> MIVSSSIVFDIFNYIGIVAFA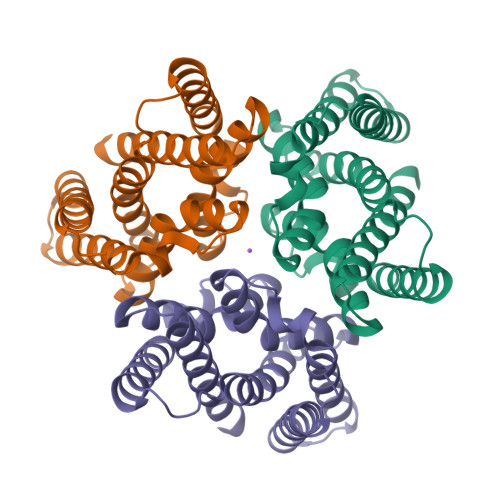ISGAIKAVKKGMDLLGVLVLGFSTALGGGIISNLLLGKTPPTNLIYYPYPITAFLASLATFVFYRIFTNVGKPLLYADAIGLGAFASSGASLAYSVSNNVILVVIVGAITAVGGGVIRDILSNEVPLILTREFYATTAVIGSFVYFIASDLSVPEDVALIVSFLITLILRILAMELKWELPRKKIEAAAENLYFQGLEDYKDDDDKHHHHHHHHHH> MKLLTHNLLSSHVRGVGSRGFPLRL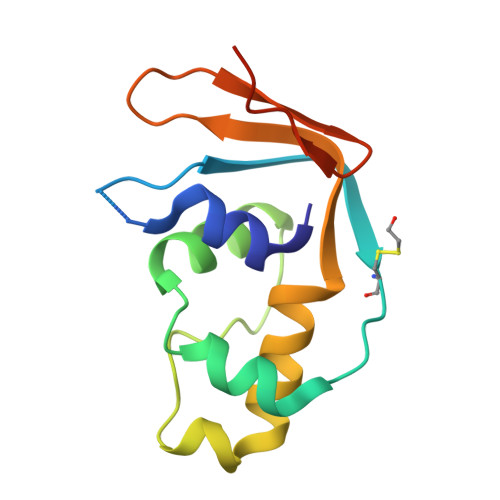QATEVRICPVEFNPNFVARMIPKVEWSAFLEAADNLRLIQVPKGPVEGYEENEEFLRTMHHLLLEVEVIEGTLQCPESGRMFPISRGIPNMLLSEEETES> QYSSNTQQGRTSIVHLFEWRWVDIALECERYLAPKGFGGVQVSPPNENVAIHNPFRPWWERYQPVSYKLCTRSGNEDEFRNMVTRCNNVGVRIYVDAVINHMCGNAVSAGTSSTCGSYFNPGSRDFPAVPYSGWDFNDGKCKTGSGDIENMNDATQVRDCRLSGLLDLALGKDYVRSKIAEYMNHLIDIGVAGFRIDASKHMWPGDIKAILDKLHNLNSNWFPEGSKPFIYQEVIDLGGEPIKSSDYFGNGRVTEFKYGAKLGTVIRKWNGEKMSYLKNWGEGWGFMPSDRALVFVDNHDNQRGHGAGGASILTFWDARLYKMAVGFMLAHPYGFTRVMSSYRWPRYFENGKDVNDWVGPPNDNGVTKEVTINPDTTCGNDWVCEHRWRQIRNMVNFRNVVDGQPFTNW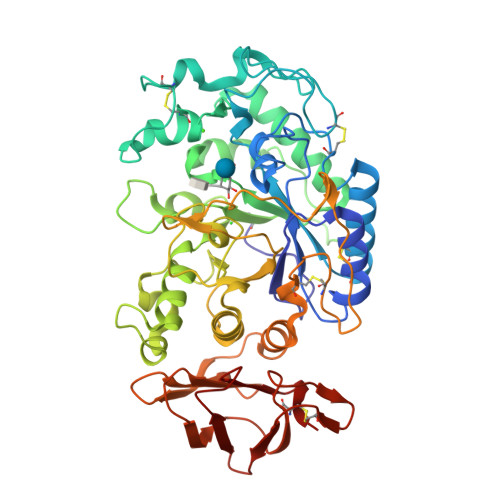YDNGSNQVAFGRGNRGFIVFNNDDWTFSLTLQTGLPAGTYCDVISGDKINGNCTGIKIYVSDDGKAHFSISNSAEDPFIAIHAESKL On the other hand, glycogen degradation requires the glycogen debranching enzyme (GDE; GlgX), which directly catalyzes the hydrolysis of α-(1→6)-linked glucose residues and the glycogen phosphorylase (GP; GlgP) to generate glucose-1-phosphate, which feeds into primary metabolism. In this study, we identify the GDE of S. venezuelae, GlgX, as a target of c-di-GMP thus uncovering a direct link between c-di-GMP and glycogen metabolism in this bacterium. We demonstrate that c-di-GMP binding stimulates GlgX-mediated glycogen breakdown and describe crystal structures of S. venezuelae GlgX, which reveal the molecular mechanism by which c-di-GMP activates GlgX. GlgX is a 79 kDa protein that contains a putative carbohydrate-binding module (CBM_48; PF02922) and alpha amylase, catalytic domain (PF00128).

We first obtained a crystal structure of the apo GlgX enzyme to 3.5 Å resolution (Methods section). The structure was refined to Rwork/Rfree values of 21.1%/27.6% and consists of three main domains, an N-terminal β-sandwich region (residues 1–145) comprised of eight β-strands and several short helices, a Central domain (residues 146–575) that harbors a α/β barrel fold similar to that found in many α-amylase enzyme structures and which consists of eight β-strands surrounded by eight α-helices. Finally, the C-terminal domain (residues 576–706) contains three β-sheets assembled from eight β-strands. Strikingly, in the structure, a c-di-GMP monomer is bound at each end of an antiparallel GlgX dimer. Note, a similar dimer was observed in the crystal packing of the apo GlgX. Insight into this question was provided by an overlay of the c-di-GMP bound S. venezuelae GlgX onto the apo structure. This overlay revealed that significant conformational changes occur upon c-di-GMP binding in several regions of the structure that are transmitted to the active site region. Specifically, c-di-GMP binding leads to a restructuring of two loops formed by residues 432–442 and 579–593 within the C-domain region bound by the second messenger. This results in concomitant conformational changes in residues 377–396 and residues 341–355. Importantly, residues 377–396 and 341–355 contain the key catalytic residues, Glu378 and Asp342. Hence, the conformational changes lead to a restructuring of the active site pocket.

>GSHMQVWPGQAYPLGATYDGAGTNFAVFSEAAHRIELCLLHDDGSETAVELRETDAFVRHAYLPGVMPGQRYGFRVHGPYAPERGLRCNAAKLLLDPYARAVSGRVRWGEAVYGYPFGRPDARNDLDSAPDTMTSVVVNPYFDWGDDRRPRTEYHHTVIYEAHVKGLTMLHPDLPEELRGTYAGLAHPSVIGHLRELGVTALELMPVHQFVNDHRLVDAGLSNYWGYNTIGFFAPHNAYASWGDRGQQVLEFKSAVRALHQAGIEVILDVVYNHTAEGNHLGPTLSMRGLDNPSYYRLADDPRYYMDTTGTGNSLLMRSPHVLQLIMDSLRYWVTEMHVDGFRFDLAATLARQFHEVDRLSSFFDLVQQDPVVSQVKLIAEPWDVGEGGYQVGNFPPLWTEWNGKYRDCVRDLWRGEPRTLAEFASRLTGSSDLYQDDGRRPLASVNFVTCHDGFTLRDLVSYNEKRNEANGEGNRDGENYNRSWNCGEEGETEDVGITELRARQMRNFLATLMLSQGVPMLSHGDEFGRTQGGNNNAYCQDNEVSWVRWPKENSEAEATLLRFTRSMVRLRREHPVFRRRRFFHGRPVEGTHDELTDIAWFTPEGEEMTSRDWQAAHAQALTVFLNGNAISEPGTQGERIADDSFLLMFNASAKELEFVVPDSHGRYWRMVVDTSDPEGMPPQQGPELAGGERVTLAPLSLTVLRRPA[12x]>[2x]GSHMGDKEKETLFKDYLNLIVV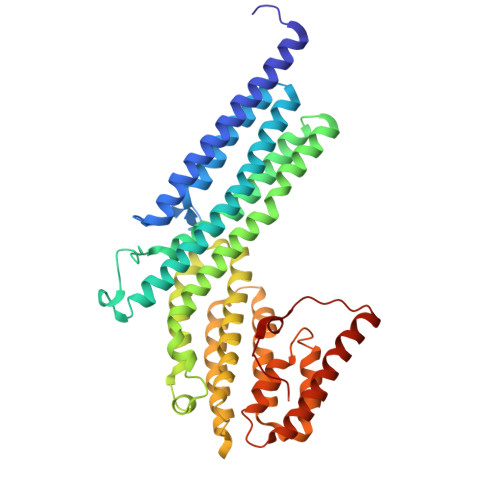KMTEWIGNLEKAEFDVFLERSTPPHSDSDGLLFLDGTKTCFQMFTQQVEVAAGTNQAKILVGVVERFSDLLTKRQKNWISKISEEIKKQINYNHKYDIDPESITPEDECPGGLVEYLIAVSNDQMKAADYAVAISSKYGKLVSKVYEKQITNHLEGTLDGFAEVAQCSSLGLITLMFDDLRKPYQEIFSKTWYMGSQAQQIADTLDEYLLDIKPQMNSVLFVNFIDNVIGETIIKFLTALSFEHSFKNKNNKFLEAMKRDFEIFYQLFVKVLDGNESKDTLITQNFTVMEFFMDLSCEPIDSILDIWQKYLEVYWDSRIDLLVGILKCRKDVSSSERKKIVQQATEMLHEYRRNMEANGVDREPTLMRRFVLEFEKQ>MNVSAESGAPRRAGQRHEVGLAQLPPAPPTTVAVIEGLATGTPRRVVNQSDAADRVAEL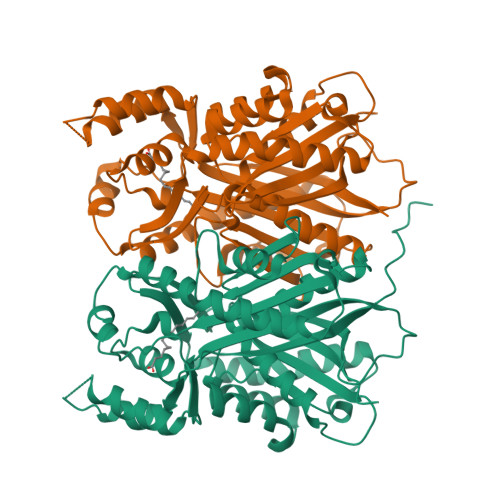FLDPGQRERIPRVYQKSRITTRRMAVDPLDAKFDVFRREPATIRDRMHLFYEHAVPLAVDVSKRALAGLPYRAAEIGLLVLATSTGFIAPGVDVAIVKELGLSPSISRVVVNFMGCAAAMNALGTATNYVRAHPAMKALVVCIELCSVNAVFADDINDVVIHSLFGDGCAALVIGASQVQEKLEPGKVVVRSSFSQLLDNTEDGIVLGVNHNGITCELSENLPGYIFSGVAPVVTEMLWDNGLQISDIDLWAIHPGGPKIIEQSVRSLGISAELAAQSWDVLARFGNMLSVSLIFVLETMVQQAESAKAISTGVAFAFGPGVTVEGMLFDIIRR[4x]(2S,4R)-2-(2-{[3-(4-fluoro-3-methylphenyl)propyl](methyl)amino}ethyl)-4-(4-fluorophenyl)-N-hydroxy-4-methoxybutanamide | 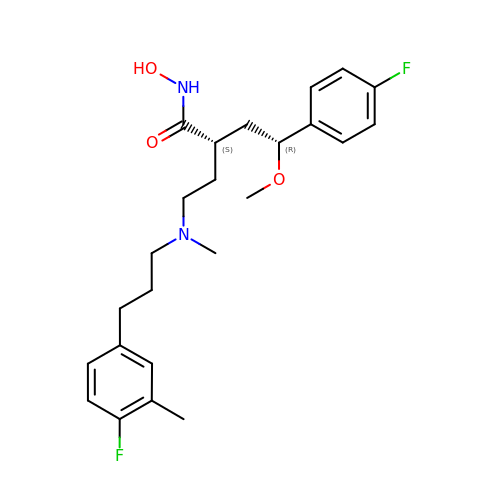C24 H32 F2 N2 O3 | VNXRIINFDPLDNI-NZQKXSOJSA-N>QAEEWYFGKITRRESERLLLNPENPRGTFLVRESETTKGAYCLSVSDFDNAKGLNVKHYKIRKLDSGGFYITSRTQFSSLQQLVAYYSKHADGLCHRLTNV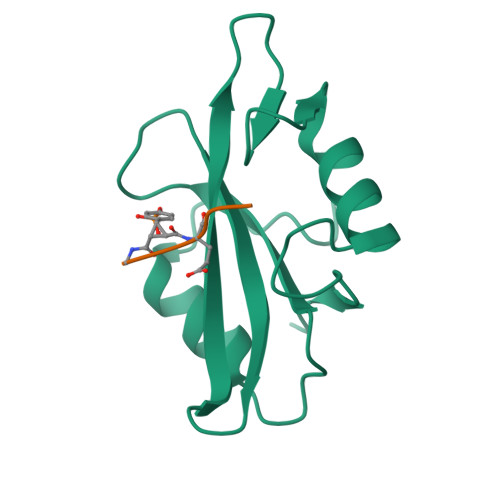CPTSK[2x]> GSLHMIDYKEIEVEEVVGRGAFGVVCKAKWRAKDVAIKQIESESERKAFIVELRQLSRVNHPNIVKLYGACLNPVCLVMEYAEGGSLYNVLHGAEPLPYY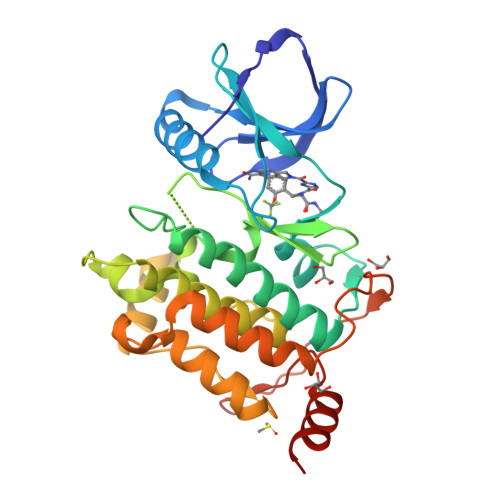TAAHAMSWCLQCSQGVAYLHSMQPKALIHRDLKPPNLLLVAGGTVLKICDFGTACDIQTHMTNNKGSAAWMAPEVFEGSNYSEKCDVFSWGIILWEVITRRKPFDEIGGPAFRIMWAVHNGTRPPLIKNLPKPIESLMTRCWSKDPSQRPSMEEIVKIMTHLMRYFPGADEPLQYPCQHSLPPGEDGRVEPYVDFAEFYRLWSVDHGEQSVVTAP Formation of active HIV-1 reverse transcriptase (RT) proceeds via a structural maturation process that involves subdomain rearrangements and formation of an asymmetric p66/p66′ homodimer. The viral RNA codes for a p66 protein that forms an asymmetric homodimer in which the RNase H domain in one subunit becomes destabilized, leading to subsequent unfolding and proteolysis in order to form the active p66/p51 heterodimer. We utilized the isolated polymerase domain, p51, rather than p66, since the initial subdomain rearrangements are largely limited to this domain. Two different fingers/palm/connection (FPC) subdomain constructs containing the same interfaces that are present in the monomers and in the p51 subunit of the RT heterodimer were investigated using both NMR spectroscopy and X-ray crystallography.

In addition, we relied on our previous strategy of deleting a disordered palm subdomain C-terminal segment (Lys219—Met230, referred to as the palm loop or PL) in order to block the metamorphic transition to p51* and, consequently, dimer formation. The fingers/palm/connection FPC1 contains the same palm subdomain deletion used in our previous studies of the p51 monomer. The globular fingers, palm, and connection subdomains of FPC1 overlay well with those of both the p51 subunit of RT and the p51 monomer. Although crystal structures were obtained for both FPC1 and FPC2, the FPC constructs did not crystallize readily, perhaps due to the dynamic behavior of several loops.

> SDHHHHHHGPISPIETVPVKLKPGMDGPKVKQWPLTEEKIKALVEICTEMEKEGKISKIGPENPYNTPVFAIKKKDSTKWRKLVDFRELNKRTQDFWEVQLGIPHPAGLKKKKSVTVLDVGDAYFSVPLDEDFRKYTAFTIPSINNETPGIRYQYNVLPQGWKGSPAIFQSSMTKILEPFKKQNPDIVIYQYMDDLYVGSDLEIGQHRTKIEELRQHLLRWGLTTPDGYELHPDKWTGSGSGGYDPSKDLIAEIQKQGQGQWTYQIYQEPSKNLKTGKYARKRGAHTNDVKQLTEAVQKITTESIVIWGKTPKFKLPIQKETWETWWTEYWQATWIPEWEFVN>[6x]GAHMAGRSMQAARCPTDELSLSNCAVVSEKDYQSGQHVIVRTSPNHKYIFTLRTHPSVVPGSVAFSLPQRKWAGLSIGQEIEVALYSFDKAKQCIGTMTIEIDFLQKKNIDSNPYDTDKMAAEFIQQFNNQAFSVGQQLVFSFNDKLFGLLVKDIEAMDPSILKGEPASGKRQKIEVGLVVGNSQVAFEKAENSSLNLIGKAKTKENRQSIINPDWNFEKMGIGGLDKEFSDIFRRAFASRVFPPEIVEQMGCKHVKGILLYGPPGCGKTLLARQIGKMLNAREPKVVNGPEILNKYVGESEANIRKLFADAEEEQRRLGANSGLHIIIFDEIDAICKQRGSMAGSTGVHDTVVNQLLSKIDGVEQLNNILVIGMTNRPDLIDEALLRPGRLEVKMEIGLPDEKGRLQILHIHTARMRGHQLLSADVDIKELAVETKNFSGAELEGLVRAAQSTAMNRHIKASTKVEVDMEKAESLQVTRGDFLASLENDIKPAFGTNQEDYASYIMNGIIKWGDPVTRVLDDGELLVQQTKNSDRTPLVSVLLEGPPHSGKTALAAKIAEESNFPFIKICSPDKMIGFSETAKCQAMKKIFDDAYKSQLSCVVVDDIERLLDYVPIGPRFSNLVLQALLVLLKKAPPQGRKLLIIGTTSRKDVLQEMEMLNAFSTTIHVPNIATGEQLLEALELLGNFKDKERTTIAQQVKGKKVWIGIKKLLMLIEMSLQMDPEYRVRKFLALLREEGASPLDFD;>GSMDTSGKQAEAMALLAEAERKVKNSQSFFSGLFGGSSKIEEACEIYARAANMFKMAKNWSAAGNAFCQAAQLHLQLQSKHDAATCFVDAGNAFKKADPQEAINCLMRAIEIYTDMGRFTIAAKHHISIAEIYETELVDVEKAIAHYEQSADYYKGEESNSSANKCLLKVAGYAAQLEQYQKAIDIYEQVGTSAMDSPLLKYSAKDYFFKAA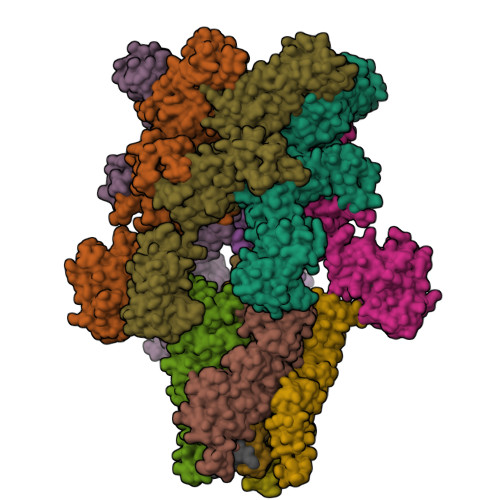LCHFCIDMLNAKLAVQKYEELFPAFSDSRECKLMKKLLEAHEEQNVDSYTESVKEYDSISRLDQWLTTMLLRIKKTIQGDEEDLR[4x];> GSNRRLQQTQAQVDEVVDIMRVNVDKVLERDQKLSELDDRADALQAGASQFETSAAKLKRKYW;> MALSEIETRHSEIIKLENSIRELHDMFMDMAMLVESQGEMIDRIEYNVEHAVDYVERAVSDTKKAVK;> RADQLADESLESTRRMLQLVEESKDAGIRTLVMLDEQGEQLDRVEEGMNHINQDMKEAEKNLKDLGKFCGLCVCPCNKLKSSDAYKKAWGNNQDGVVASQPARVVDEREQMAISGGFIRRVTNDARENEMDENLEQVSGIIGNLRHMALDMGNEIDTQNRQIDRIMEKADSNKTRIDEANQRATKMLG> GHSYEKYNNWETIEAWTK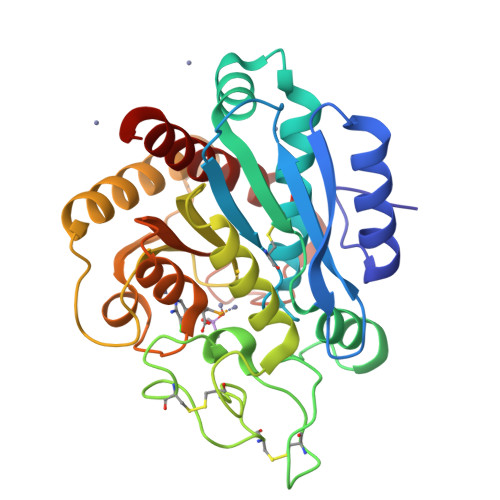QVTSENPDLISRTAIGTTFLGNNIYLLKVGKPGPNKPAIFMDCGFHAREWISHAFCQWFVREAVLTYGYESHMTEFLNKLDFYVLPVLNIDGYIYTWTKNRMWRKTRSTNAGTTCIGTDPNRNFDAGWCTTGASTDPCDETYCGSAAESEKETKALADFIRNNLSSIKAYLTIHSYSQMILYPYSYDYKLPENNAELNNLAKAAVKELATLYGTKYTYGPGATTIYPAAGGSDDWAYDQGIKYSFTFELRDKGRYGFILPESQIQATCEETMLAIKYVTNYVLGHL> ACUCGGAUGA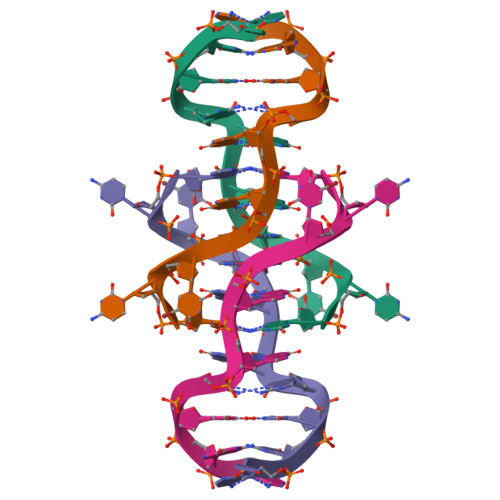T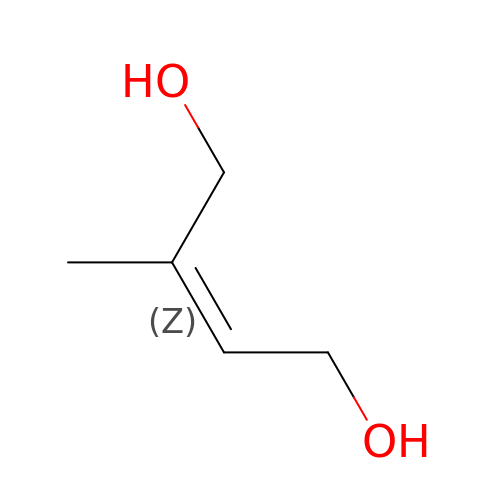(2Z)-2-methylbut-2-ene-1,4-diol | C5 H10 O2 | FLXLJBCLEUWWCG-DJWKRKHSSA-N> GPGSNLEVVHHRALVLAQIRKWLDKLMFKEAFECMRKLRINLNLIYDHNPKVFLGNVETFIKQIDSVNHINLFFTELKEEDVTKTMYPAPVTSSVYLSRDPDGNKIDLV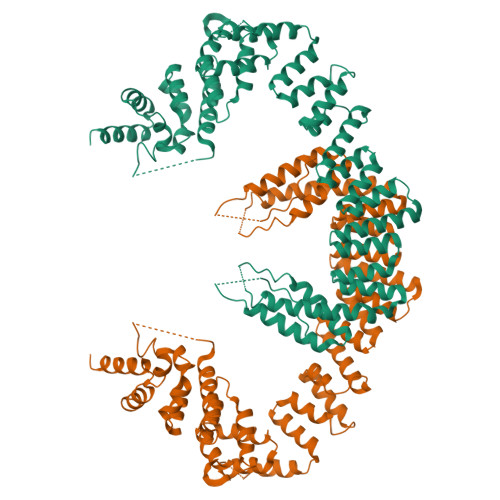CDAMRAVMESINPHKYCLSILTSHVKKTTPELEIVLQKVHELQGNAPSDPDAVSAEEALKYLLHLVDVNELYDHSLGTYDFDLVLMVAEKSQKDPKEYLPFLNTLKKMETNYQRFTIDKYLKRYEKAIGHLSKCGPEYFPECLNLIKDKNLYNEALKLYSPSSQQYQDISIAYGEHLMQEHMYEPAGLMFARCGAHEKALSAFLTCGNWKQALCVAAQLNFTKDQLVGLGRTLAGKLVEQRKHIDAAMVLEECAQDYEEAVLLLLEGAAWEEALRLVYKYNRLDIIETNVKPSILEAQKNYMAFLDSQTATFSRHKKRLLVVRELKEQAQQAGLDDEVPHGQESDLFSETSSVVSGSEMSGKYSHSNSRISARSSKNRRKAERKKHSLKEGSPLEDLALLEALSEVVQNTENLKDEVYHILKVLFLFEFDEQGRELQKAFEDTLQLMERSLPEIWTLTYQQNSATPVLGPNSTANSIMASYQQQKTSVPVLDAELFIPPKINRRTQWKLSLLD> MTDRLTQLQICLDQMTEQFCATLNYIDKNHGFERLTVNEPQMSDKHATVVPPEEFSNTIDELSTDIILKTRQINKLIDSLPGVDVSAEEQLRKIDMLQKKLVEVEDEKIEAIKKKEKLLRHVDSLIEDFVDGIANSKKSTAAA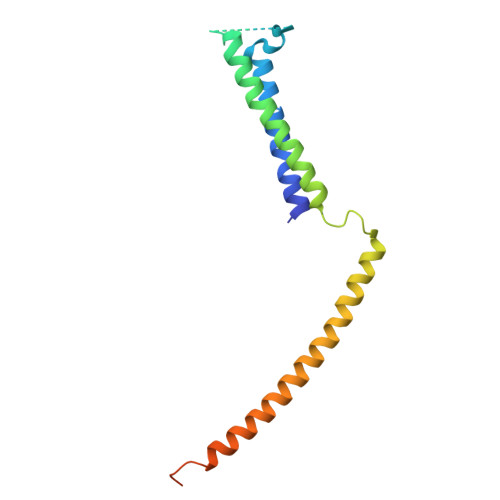LEHHHHHH>[2x]MDSFWFVQQWPPAVCSFQKSGSCPGSGLRTFTIHGLWPQQSGTS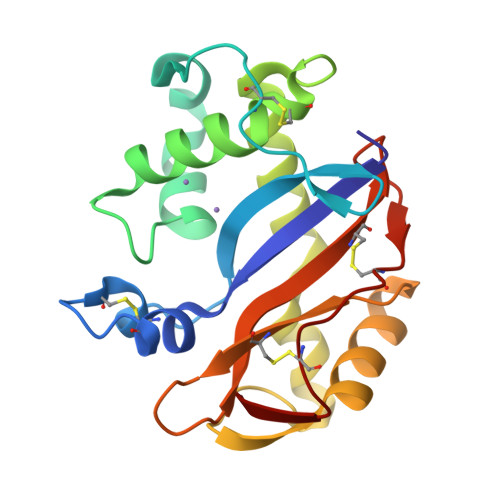LTNCPGSPFDITKISHLQSQLNTLWPTVLRANNQQFWSHEWTKHGTCSESTFNQAAYFKLAVDMRNNYDIIGALRPHAAGPNGRTKSRQAIKGFLKAKFGKFPGLRCRTDPQTKVSYLVQVVACFAQDGSTLIDCTRDTCGANFIF> DR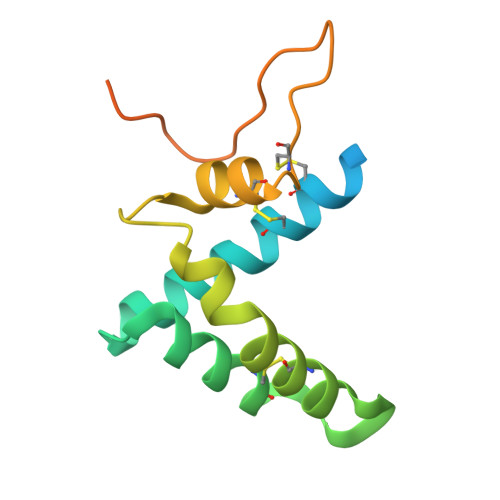HHHHHHKLSRAHDNQPGTIRSDHYTCVGCVLVVSVIEQLAQVHNSTVQASMERLCSYLPEEWVLKTACYMMVHVFGADIIKLFDKDVNADVVCHTLEFCKQEPGQPLCHLYPLPKESWKFTLEKARHIVKQSPIMKYTR> ANNLPDTQSSGPAHSKETPALTAVETGATNPLVPSDTVQTRHVIQKRTRSESTVESFFARGACVAIIEVDNDAPTKRASKLFSVWKITYKDTVQLRRKLEFFTYSRFDMEFTFVVTSNYTDANNGHALNQVYQIMYIPPGAPIPGKWNDYTWQTSSNPSVFYTYGAPPARISVPYVGIANAYSHFYDGFAKVPLAGQASTEGDSLYGAASLNDFGSLAVRVVNDHNPTKLTSKIRVYMKPKHVRVWCPRPPRAV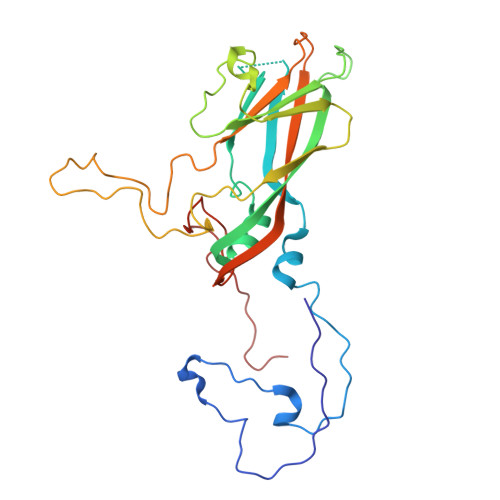PYYGPGVDYKDGLAPLPGKGLTTY>[2x]MKLQTTYPSNNYPIYVEHGAIKYIGTYLNQFDQSFLLIDEYVNQYFANKFDDILSYENVHKVIIPAGEKTKTFEQYQETLEYILSHHVTR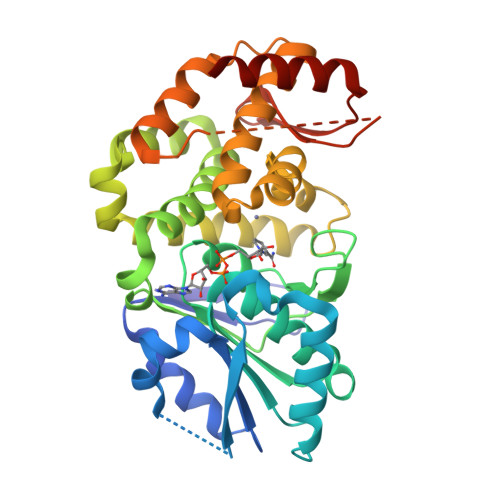NTAIIAVGGGATGDFAGFVAATLLRGVHFIQVPTTILAHDSSVGGKVGINSKQGKNLIGAFYRPTAVIYDLDFLKTLPFKQILSGYAEVYKHALLNGESATQDIEQHFKDREILQSLNGMDKYIAKGIETKLDIVVADEKEQGVRKFLNLGHTFGHAVEYYHKIPHGHAVMVGIIYQFIVANALFDSKHDISHYIQYLIQLGYPLDMITDLDFETLYQYMLSDKKNDKQGVQMVLMRQFGDIVVQHVDQLTLQHACEQLKTYFK>[2x]MYVDRKPSLYLEDLRHDFKNSLSKFENGDEAFDTLLGFVELDHIYSSALKEIST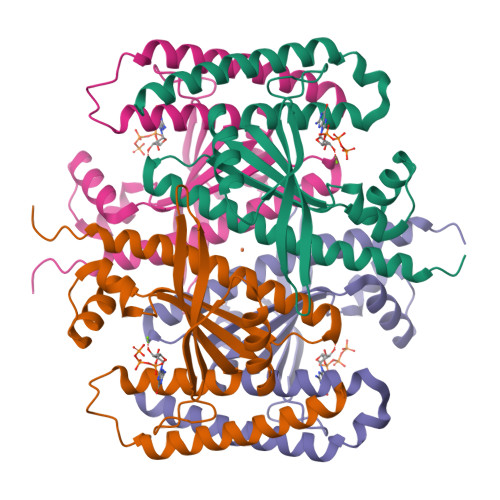KLSILDDNFNHIYKHNPIHHMERRVKEMRSLIEKLNRKGLQISAETAKEHILDIAGIRVVCNYLDDIYLIEEMLLKQEDVQLIKRKDYIQHPKENGYRSLHIVVSIPVFLAERVEVLPVEIQIRTIGMDMWASLEHKIRYKNNAETEKYRDLLKECATEITEVEDKLQQIHSEITEGHHHHHH>[2x]MTKFSGNELRAELYRRAFLSYSVAPGALGMFGRSLLAKGARAEALANGTVMSGSHWGVFTATVENGRATAFTPWEKDPHPSPMLAGVLDSIYSPTRIKYPMVRREFLEKGVNADRSTRGNGDFVRVSWDQALDLVAAEVKRVEETYGPEGVFGGSYGWKSPGRLHNCTTLLRRMLTLAGGYVNGAGDYSTGAAQVIMPHVVGTLEVYEQQTAWPVLAENTEVMVFWAADPIKTSQIGWVIPEHGAYPGLEALKAKGTKVIVIDPVRTKTVEFFGAEHITPKPQTDVAIMLGMAHTLVAEDLYDKDFIANYTSGFDKFLPYLDGETDSTPKTAEWAEGISGVPAETIKELARLFESKRTMLAAGWSMQRMHHG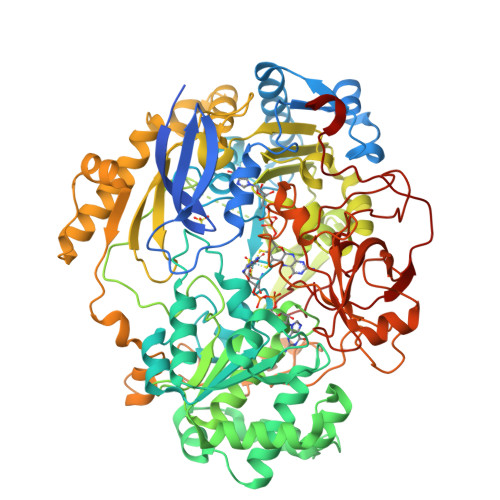EQAHWMLVTLASMLGQIGLPGGGFGLSYHYSGGGTPSTSGPALAGITDGGAATKGPEWLAASGASVIPVARVVDMLENPGAEFDFNGTRSKFPDVKMAYWVGGNPFVHHQDRNRMVKAWEKLETFVVHDFQWTPTARHADIVLPATTSYERNDIETIGDYSNTGILAMKKIVEPLYEARSDYDIFAAVAERLGKGAEFTEGKDEMGWIKSFYDDAAKQGKAAGVQMPAFDAFWAEGIVEFPVTDGADFVRYASFREDPLLNPLGTPTGLIEIYSKNIEKMGYDDCPAHPTWMEPLERLDGPGAKYPLHIAASHPFNRLHSQLNGTVLREGYAVQGHEPCLMHPDDAAARGIADGDVVRVHNDRGQILTGVKVTDAVMKGVIQIYEGGWYDPSDVTEPGTLDKYGDVNVLSADIGTSKLAQGNCGQTVLAEVEKYTGPAVTLTGFVAPKAAE> AATHLEVARGKRAALFFAAVAIVLGLPLWWKTTETYRASLPYSQISGLNALQLRLMVPVTVVFTRESVPLDDQAKLPFTVVHEREIPLKYKMKIKCRFQKAYRRALDHEEEALSSGSVQEAEAMLDEPQEQAEGSLTVYVISEHSSLLPQDMASYIGPKRT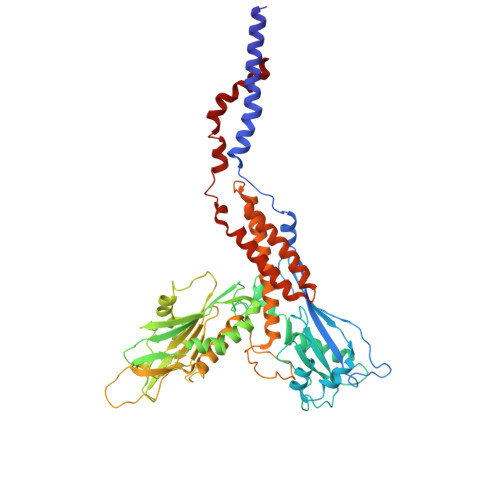AVVRGIMHREAFNIIGRRIVQVAQAMSLTEDVLAAALADHLPEDKWSAEKRRPLKSSLGYEITFSLLNPDPKSHDVYWDIEGAVRRYVQPFLNALGAAGNFSVDSQILYYAMLGVNPRFDSASSSYYLDMHSLPHVINPVESRLGSSAASLYPVLNFLLYVPELAHSPLYIQDKDGAPVATNAFHSPRWGGIMVYNVDSKTYNASVLPVRVEVDMVRVMEVFLAQLRLLFGIAQPQLPPKCLLSGPTSEGLMTWELDRLLWARSVENLATATTTLTSLAQLLGKISNIVIKDDVASEVYKAVAAVQKSAEELASAHLASAFVASQEAVTSSELAFFDASLLHLLYFPDDQKFAIYIPLFLPMAVPILLSLVK>[2x]MKAPVRVAVTGAAGQIGYSLLFRIAAGEMLGKDQPVILQLLGSERSFQALEGVVMELEDCAFPLLAGLEATDDPKVAFKDADYALL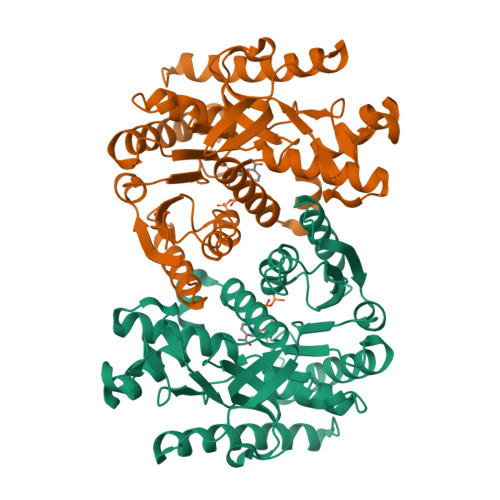VGAAPRKAGMERRDLLQVNGKIFTEQGRALAEVAKKDVKVLVVGNPANTNALIAYKNAPGLNPRNFTAMTRLDHNRAKAQLAKKTGTGVDRIRRMTVWGNHSSTMFPDLFHAEVDGRPALELVDMEWYEKVFIPTVAQRGAAIIQARGASSAASAANAAIEHIRDWALGTPEGDWVSMAVPSQGEYGIPEGIVYSFPVTAKDGAYRVVEGLEINEFARKRMEITAQELLDEMEQVKALGLI>[2x]GPDSMLADSFEQEASREVDASKGLTNSETLQVEQDGKVRLSHQVRHQVALPPNYDYTPIAEHKRVNEARTYPFTLDPFQDTAISCIDRGESVLVSAHTSAGKTVVAEYAIAQSLKNKQRVIYTSPIKALSNQKYRELLAEFGDVGLMTGDITINPDAGCLVMTTEILRSMLYRGSEVMREVAWVIFDEVHYMRDKERGVVWEETIILLPDKVRYVFLSATIPNAMEFAEWICKIHSQPCHIVYTNFRPTPLQHYLFPAHGDGIYLVVDEKSTFREENFQKAMASISNQIGDDPNSTDSRGKKGQTYKGGSAKGDAKGDIYKIVKMIWKKKYNPVIVFSFSKRDCEELALKMSKLDFNSDDEKEALTKIFNNAIALLPETDRELPQIKHILPLLRRGIGIHHSGLLPILKEVIEILFQEGFLKVLFATETFSIGLNMPAKTVVFTSVRKWDGQQFRWVSGGEYIQMSGRAGRRGLDDRGIVIMMIDEKMEPQVAKGMVKGQADRLDSAFHLGYNMILNLMRVEGISPEFMLEHSFFQFQNVISVPVMEKKLAELKKDFDGIEVEDEENVKEYHEIEQAIKGYREDVRQVVTHPANALSFLQPGRLVEISVNGKDNYGWGAVVDFAKRINKRNPSAVYTDHESYIVNVVVNTMYIDSPV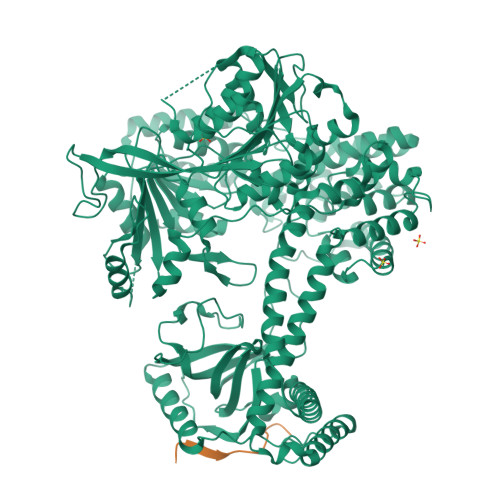NLLKPFNPTLPEGIRPAEEGEKSICAVIPITLDSIKSIGNLRLYMPKDIRASGQKETVGKSLREVNRRFPDGIPVLDPVKNMKIEDEDFLKLMKKIDVLNTKLSSNPLTNSMRLEELYGKYSRKHDLHEDMKQLKRKISESQAVIQLDDLRRRKRVLRRLGFCTPNDIIELKGRVACEISSGDELLLTELIFNGNFNELKPEQAAALLSCFAFQERCKEAPRLKPELAEPLKAMREIAAKIAKIMKDSKIEVVEKDYVESFRHELMEVVYEWCRGATFTQICKMTDVYEGSLIRMFKRLEELVKELVDVANTIGNSSLKEKMEAVLKLIHRDIVSAGSLYL;>GPDSMALFHVDVEGDEILKNKLIKRKQIKKVLKSKEIL[2x]> MSASFVPNGASLEDCHCNLFCLADLTGIKWKKYVWQGPTSAPILFPVTEEDPILSSFSRCLKADVLGVWRRDQRPGRRELWIFWWGEDPSFADLIHHDLSEEEDGVWENGLSYECRTLLFKAVHNLLERCLMNRNFVRIGKWFVKPYEKDEKPINKSEHLSCSFTFFLHGDSNVCTSVEINQHQPVYLLSEEHITLAQQSNSPFQVILCPFGLNGTLTGQAFKMSDSATKKLIGEWKQFYPISCCLKEMSEEKQEDMDWEDDSLAAVEVLVAGVRMIYPACFVLVPQSDIPTPSPVGSTHCSSSCLGVHQVPASTRDPAMSSVTLTPPTSPEEVQTVDPQSVQKWVKFSSVSDGFNSDSTSHHGGKIPRKLANHVVDRVWQECNMNRAQNKRKYSASSGGLCEEATAAKVASWDFVEATQRTNCSCLRHKNLKSRNAGQQGQAPSLGQQQQILPKHKTNEKQEKSEKPQKRPLTPFHHRVSVSDDVGMDADSASQRLVISAPDSQVRFSNIRTNDVAKTPQMHGTEMANSPQPPPLSPHPCDVVDEGVTKTPSTPQSQHFYQMPTPDPLVPSKPMEDRIDSLSQSFPPQYQEAVEPTVYVGTAVNLEEDEANIAWKYYKFPKKKDVEFLPPQLPSDKFKDDPVGPFGQESVTSVTELMVQCKKPLKVSDELVQQYQI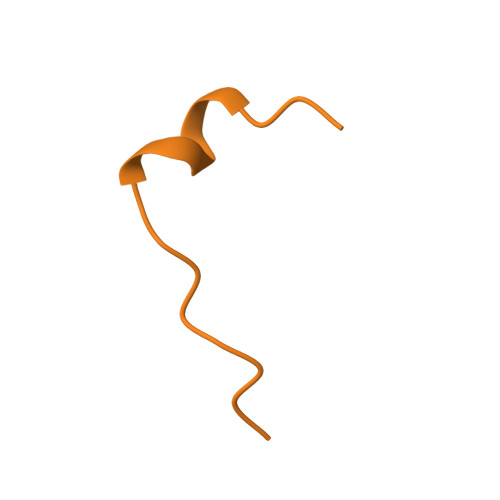KNQCLSAIASDAEQEPKIDPYAFVEGDEEFLFPDKKDRQNSEREAGKKHKVEDGTSSVTVLSHEEDAMSLFSPSIKQDAPRPTSHARPPSTSLIYDSDLAVSYTDLDNLFNSDEDELTPGSKKSANGSDDKASCKESKTGNLDPLSCISTADLHKMYPTPPSLEQHIMGFSPMNMNNKEYGSMDTTPGGTVLEGNSSSIGAQFKIEVDEGFCSPKPSEIKDFSYVYKPENCQILVGCSMFAPLKTLPSQYLPPIKLPEECIYRQSWTVGKLELLSSGPSMPFIKEGDGSNMDQEYGTAYTPQTHTSFGMPPSSAPPSNSGAGILPSPSTPRFPTPRTPRTPRTPRGAGGPASAQGSVKYENSDLYSPASTPSTCRPLNSVEPATVPSIPEAHSLYVNLILSESVMNLFKDCNFDSCCICVCNMNIKGADVGVYIPDPTQEAQYRCTCGFSAVMNRKFGNNSGLFLEDELDIIGRNTDCGKEAEKRFEALRATSAEHVNGGLKESEKLSDDLILLLQDQCTNLFSPFGAADQDPFPKSGVISNWVRVEERDCCNDCYLALEHGRQFMDNMSGGKVDEALVKSSCLHPWSKRNDVSMQCSQDILRMLLSLQPVLQDAIQKKRTVRPWGVQGPLTWQQFHKMAGRGSYGTDESPEPLPIPTFLLGYDYDYLVLSPFALPYWERLMLEPYGSQRDIAYVVLCPENEALLNGAKSFFRDLTAIYESCRLGQHRPVSRLLTDGIMRVGSTASKKLSEKLVAEWFSQAADGNNEAFSKLKLYAQVCRYDLGPYLASLPLDSSLLSQPNLVAPTSQSLITPPQMTNTGNANTPSATLASAASSTMTVTSGVAISTSVATANSTLTTASTSSSSSSNLNSGVSSNKLPSFPPFGSMNSNAAGSMSTQANTVQSGQLGGQQTSALQTAGISGESSSLPTQPHPDVSESTMDRDKVGIPTDGDSHAVTYPPAIVVYIIDPFTYENTDESTNSSSVWTLGLLRCFLEMVQTLPPHIKSTVSVQIIPCQYLLQPVKHEDREIYPQHLKSLAFSAFTQCRRPLPTSTNVKTLTGFGPGLAMETALRSPDRPECIRLYAPPFILAPVKDKQTELGETFGEAGQKYNVLFVGYCLSHDQRWILASCTDLYGELLETCIINIDVPNRARRKKSSARKFGLQKLWEWCLGLVQMSSLPWRVVIGRLGRIGHGELKDWSCLLSRRNLQSLSKRLKDMCRMCGISAADSPSILSACLVAMEPQGSFVIMPDSVSTGSVFGRSTTLNMQTSQLNTPQDTSCTHILVFPTSASVQVASATYTTENLDLAFNPNNDGADGMGIFDLLDTGDDLDPDIINILPASPTGSPVHSPGSHYPHGGDAGKGQSTDRLLSTEPHEEVPNILQQPLALGYFVSTAKAGPLPDWFWSACPQAQYQCPLFLKASLHLHVPSVQSDELLHSKHSHPLDSNQTSDVLRFVLEQYNALSWLTCDPATQDRRSCLPIHFVVLNQLYNFIMNML> MAAGKEVGRLSIKVTPDLDGFYRELKAAVEAAEKMKVHIPVEPDMGNFRQEVAASTAGMSTRVKVQADVDRGLLDRLSNSLSGMKAPSFGSGINPTGYMLILGAAAALTPLIAGSLGAISAALLTLPGLIAAVAVPIGALALGIDGFKRAAERLKPAFDGLKESMSAAVENQFGPVFDQLGKAIPTLAANLPKVTQGMADVAKSIVDSVTSGEGLGRIESLISNIGAAISRSAPGLTSFVDGLLNLAEKFSGKLPAIADWINRTGESFSKWVTDFTTAGPDGVSKFDNAMSGLGDTLQMLGGGLVDILNKSLEFFSDPQKIQSFKAELDGLIASISTLVDLINSLAAAFSKVPGLSDGEANGVMDFAPIQIQGAIELIKQIPTAWEGVKLKAAEVWNSIPTMAATAIASIRATLATLPGLLSGIWTTVTASASSAFATIGAAVSAGARSVVNTAGNIFRSMGSVIANAFSAAVSAVQTAFSQMVSAAASGAQQVVAEVQALGGKIAAAAGNFGSILVAAGKALMDGLLSGIKAGLSAVLDFASGIAAKIAAVKGPLPKDRKELIPAGEALMEGLGTGIENGLDPVLDRAREIAKQIFSAFKETFGTAPTSLAFNLGSMQGDLSGLQTSLESTATASRDLTSSLTAPTAELASGSSLLGDDVKDQLDELKLAYDQLELQRKQLKVQKNEAGSKEDKAAIQDKIDALQAEKDKLA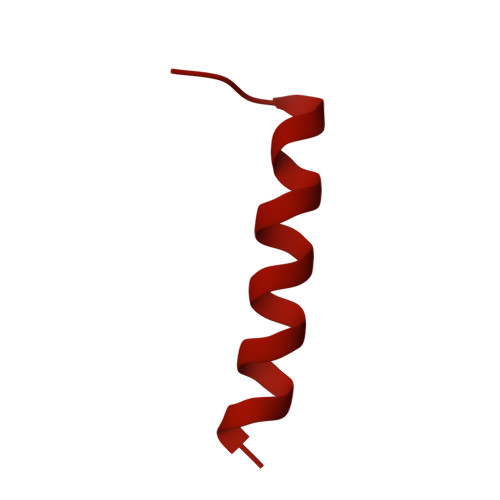YQKDQLKIQQKQTGEMGEQKTLAQFLGEQIASTWQQGTDAVAGFARSNLDQAMSDLGIGGGAITNGLNAGLDWGVQALGNAVNIQVNSVDDAIAVKNNEVNKQALTYTRR> MQVIRKHLAQKGLFNPFLFNRFSTQQDITSVPGDKPPAIEDSIHGKYAGVLFSSASSNKSLNKVAEDMKYFNQLYKESEVFKSFLNNVSLKRNQQRDIISALGKTNFNPATNNLLETLIENKRLDSLPKIAEKYMDYYRILNKQESITIISAQELTAA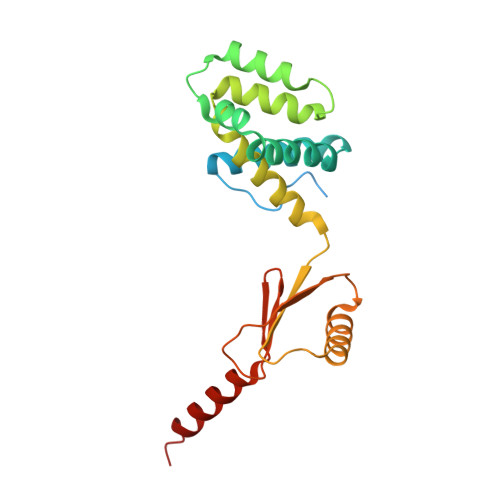EKQKVEQGLKKGNANVQFTVVYQVDPAILGGLQMYSGNNFLDCSLLSRVNKLKTEIAKISF>[2x]CUGC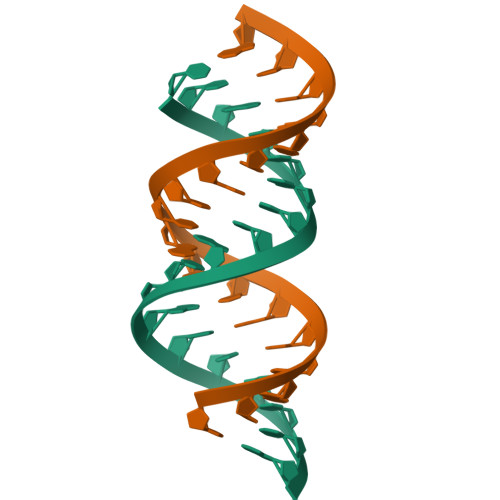UGCUGCUGCUGCUG4-hydroxy-2-oxoglutarate (HOG) aldolase is a unique enzyme in the hydroxyproline degradation pathway catalyzing the cleavage of HOG to pyruvate and glyoxylate. The crystal structures of the apoenzyme and pyruvate-Schiff base intermediate complex are the first for any HOGA enzyme to date and reveal a tetrameric structure composed of a dimer of dimers as well as the identity of active site residues. As mentioned briefly above, the crystallographic symmetry of the hHOGA crystals generate a tetrameric assembly containing a dimer of dimers. Residues 26–259 form an (α/β)8 TIM barrel domain, while residues 260–327 form a three-helical bundle at the C-terminus.

The inclusion of 10 mM pyruvate during crystallization improved diffraction substantially and allowed for in-house data collection to 1.97 Å resolution. An omit Fo-Fc map contoured to 6.4 σ shows clear continuous electron density for the imine Schiff base adduct between the ε-amino group of Lys196 and pyruvate. In this binding mode, hydrogen bonding interactions are observed between the hydroxyl group of Tyr168 and the O(1B) carboxylate oxygen atom of pyruvate. Additional hydrogen bonding interactions are present between the backbone amide nitrogen atoms of Ser77 and Asn78 and the O(1B) and O(1A) atoms of pyruvate, respectively. A network between Ser77, Tyr168, and Tyr140' from the adjacent monomer is also formed. A superposition of the apoenzyme structure with the pyruvate adduct (RMSD  = 0.19 Å for Cα atoms) reveals no significant structural changes to the active site other than a water molecule within hydrogen bonding distance to Lys196. The crystal structure of hHOGA in complex with pyruvate illustrates how the highly conserved G-X-X-G-E motif fulfills the same carboxylate-binding role via two backbone amide nitrogen atoms. The Schiff base intermediate observed within the hHOGA crystal structure and the inactivity of the K196A variant support that this residue plays the same functional role in hHOGA catalysis. The crystal structure of the enzyme in complex with pyruvate has enabled the modeling of the HOG complex and led to the identification of key active site residues. No electron density was observed for the first six residues of hHOGA and the three residues remaining from the affinity tag. The final structures for the apoenzyme and Schiff base adduct exhibited Rwork/free values of 21.2/24.6% and 19.6/21.6%, respectively, and were of high overall quality, as indicated by the refinement statistics in Table 1.

> GPLGSASGEGKKVDIAGIYPPVTTPFTATAEVDYGKLEENLHKLGTFPFRGFVVQGSNGEFPFLTSSERLEVVSRVRQAMPKNRLLLAGSGCESTQATVEMTVSMAQVGADAAMVVTPCYYRGRMSSAALIHHYTKVADLSPIPVVLYSVPANTGLDLPVDAVVTLSQHPNIVGMKDSGGDVTRIGLIVHKTRKQDFQVLAGSAGFLMASYALGAVGGVCALANVLGAQVCQLERLCCTGQWEDAQKLQHRLIEPNAAVTRRFGIPGLKKIMDWFGYYGGPCRAPLQELSPAEEEALRMDFTSNGWL>MRKKISIIGAGFVGSTTAHWLAAKELGDIVLLDIVEGVPQGKALDLYEASPIEGFDVRVTGTNNYADTANSDVIVVTSGAPRKPGMSREDLIKVNADITRACISQAAPLSPNAVIIMVNNPLDAMTYLAAEVSGFPKERVIGQAGVLDAARYRTFIAMEAGVSVEDVQAMLMGGHGDEMVPLPRFSTISGIPVSEFIAPDRLAQIVERTRKGGGEIVNLLKTGSAYYAPAAATAQMVEAVLKDKKRVMPVAAYLTGQYGLNDIYFGVPVILGAGGVEKILELPL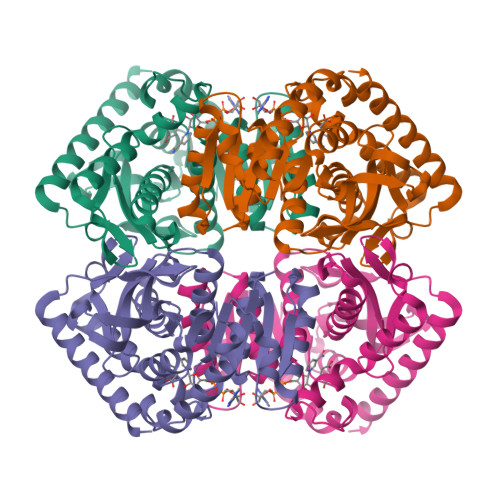NEEEMALLNASAKAVRATLDTLKSL[2x]>[2x]GMKYKAAIFDMDGTILDTSADLTSALNYAFEQTGHRHDFTV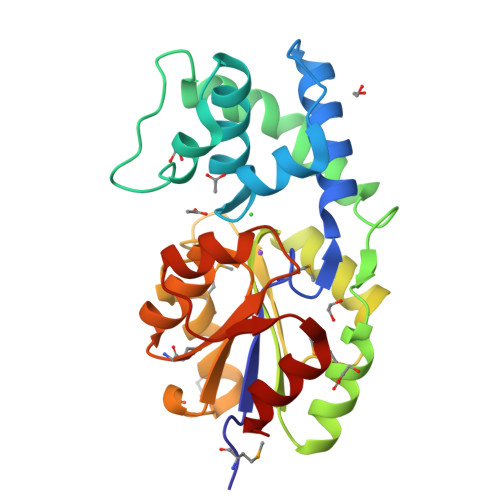EDIKNFFGSGVVVAVTRALAYEAGSSRESLVAFGTKDEQIPEAVTQTEVNRVLEVFKPYYADHCQIKTGPFPGILDLMKNLRQKGVKLAVVSNKPNEAVQVLVEELFPGSFDFALGEKSGIRRKPAPDMTSECVKVLGVPRDKCVYIGDSEIDIQTARNSEMDEIAVNWGFRSVPFLQKHGATVIVDTAEKLEEAILGE Anhydrorhodovibrin  | C41 H58 O | 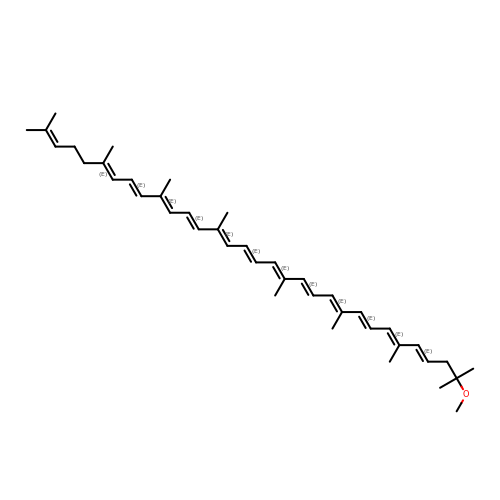OCDSWQXGIQUZCF-AGVJHCIFSA-N PENTANE-1,5-DIAMINE 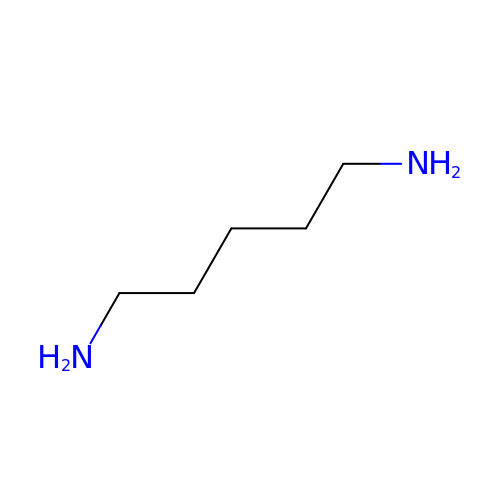| C5 H14 N2 | VHRGRCVQAFMJIZ-UHFFFAOYSA-N>[16x]MSPSVLEPQSVPTLVNVGLKAVGRNDAPVERDAR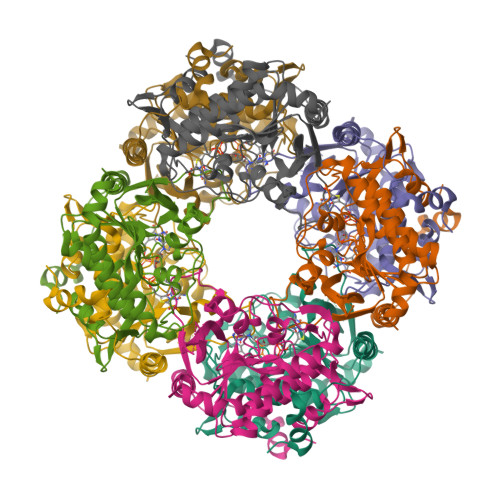GLSKPLLELMPTLGTDAFTFSPIRESTVSRAMTRRYFADLDAHAETDIVIVGAGSCGLSAAYVLSTLRPDLRITIVEAGVAPGGGAWLGGQLFSAMVMRKPADVFLDEVGVPYEDEGDYVVVKHAALFTSTVLSKVLQRPNVKLFNATTVEDLITRKHHAESSSSSDDGEAEDEAKVRIAGVVTNWTLVSMHHDDQSSMDPNTINAPVIISTTGHDGPFGAFSVKRLVSMKQMERLNGMRGLDMQSAEDAIVNNTREIVPGLIVGGMELSEIDGANRMGPTFGAMALSGVKAAHEAIRVFDLRKAQNDKC>RFLKVKNWETDVVLTDTLHLKSTLETGCTEHICMGSIMLPSQHTRKPEDVRTKDQLFPLAKEFLDQYYSSIKRFGSKAHMDRLEEVNKEIESTSTYQLKDTELIYGAKHAWRNASRCVGRIQWSKLQVFDARDCTTAHGMFNYICNHVKYATNKGNLRSAITIFPQRTDGKHDFRVWNSQLIRYAGYKQPDGSTLGDPANVQFTEICIQQGWKAPRGRFDVLPLLLQANGNDPELFQIPPELVLEVPIRHPKFDWFKDLGLKWYGLPAVSNMLLEIGGLEFSACPFSGWYMGTEIGVRDYCDNSRYNI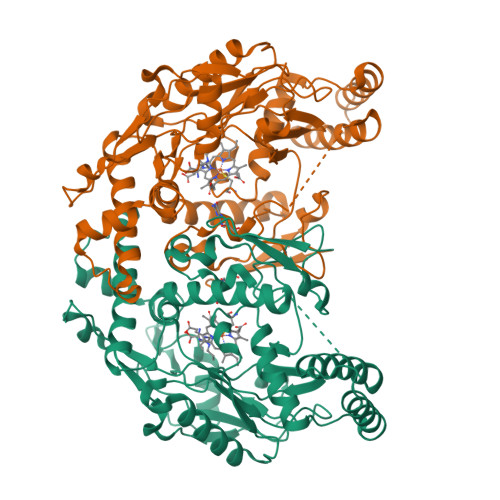LEEVAKKMDLDMRKTSSLWKDQALVEINIAVLYSFQSDKVTIVDHHSATESFIKHMENEYRCRGGCPADWVWIVPPMSGSITPVFHQEMLNYRLTPSFEYQPDPWNTHVWK[2x]N-[(2S,3R)-3-hydroxy-1-(hydroxyamino)-1-oxobutan-2-yl]biphenyl-4-carboxamide | C17 H18 N2 O4 | 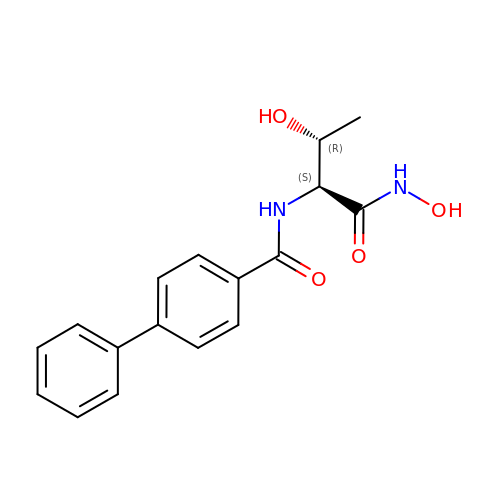AXQUTBMFDJGETC-ABAIWWIYSA-N> MAAIPPDSWQPPNVYLETSMGIIVLELYWKHAPKTCKNFAELARRGYYNGTKFHRIIKDFMIQGGDPTGTGRGGASIYGKQFEDELHPDLKFTGAGILAMANAGPDTNGSQFFVTLAPTQWLDGKHTIFGRVCQGIGMVNRVGMVETNSQDRPVDDVKIIKAYPSG;> ALLVTAGLVLA

Peptidyl-prolyl isomerase like 1 (PPIL1) is a cyclophilin and belongs to the so-called Prp19-related proteins. PPIL1 is a single domain cyclophilin and has been found to interact with the Ski-interacting protein (SKIP, also referred to as hPrp45, SNW domain-containing protein 1, nuclear receptor coactivator NCoA-62). Peptidyl-prolyl cis/trans isomerases (PPIases, E.C. 5.1.2.8) catalyze the isomerization of peptide bonds that precede a proline residue and can thereby facilitate folding of their substrate proteins. Second, PPIL1 can interact with the SKIP protein without involving its PPIase active site.

The crystal structure of PPIL1 in complex with the inhibitor cyclosporine A (CsA) was obtained at a resolution of 1.15 Å and exhibited two bound Cd2+ ions that enabled SAD phasing. The final model comprises full-length PPIL1 protein (except the very N-terminal Met) bound to CsA without any geometry violations and with good R-factors. PPIL1 exhibits the canonical cyclophilin fold comprising an eight-stranded antiparallel β-sheet capped on both sides by α-helices. All CsA-contacting residues of PPIL1 are conserved and exhibit the same side chain rotamers as observed for CypA in complex with CsA, rendering the active site geometry essentially identical to CypA and other CypA-type cyclophilins. The structure of the PPIL1·CsA complex contains two Cd2+ ions in an asymmetric unit. Both ions are coordinated by the PPIL1 protein and water molecules such that contacts between two neighboring PPIL1 molecules in the crystal lattice are established. [1] were able to pinpoint a number of PPIL1 surface-exposed residues that undergo chemical shift perturbations upon titration with SKIP59–129. Strikingly, these residues (highlighted in Figure 4B) involve the residues His87, Asp89 and Cys133, which coordinate Cd2+ ions in the present crystal structure. Cd2+ ions are directly involved in crystal packing and it appears, thus, that Cd2+-mediated crystal packing has excluded the SKIP peptide from the crystals. The PPIL1·CsA crystal structure exhibits a generally more compact shape compared to a previously published NMR structure ensemble of PPIL1. In particular, the N-terminus of the protein is not disordered as reported for the NMR structure.> HMEMSWPYPLRSRFDPQVPEEDIDYSMTSPLNSDGSNFPCKGYQTNTPWRATAQYTAGQTYNMTITGSATHGGGSCQLSLSYDNG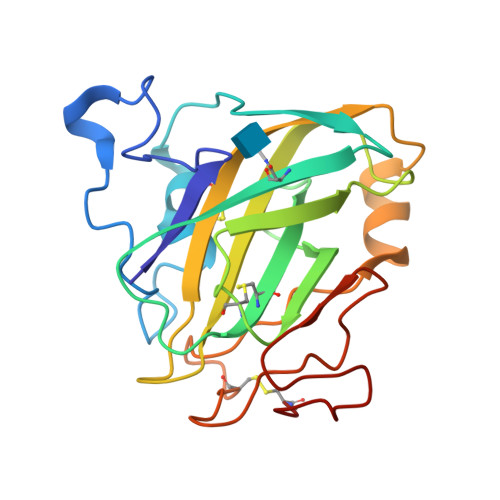KTFKVIQSMEGGCPLVSKYNFKIPGDVANGQALFAWTWYNLIGNRELYMNCADVVISGGTGTPSSFESAYPDLFVANVGNGCSTVEGRETVFANPGDQVIYGGTVTPSSPAFPICH> GARLQEIYNRMDPRAQTPVPGKGPFGREELLRRKLIHDGCLLWKTATGRFKDVLVLLMTDVLVFLQEKDQKYIFPTLDKPSVVSLQNLIVRDIANQEKGMFLISAAPPEMYEVHTASRDDRSTW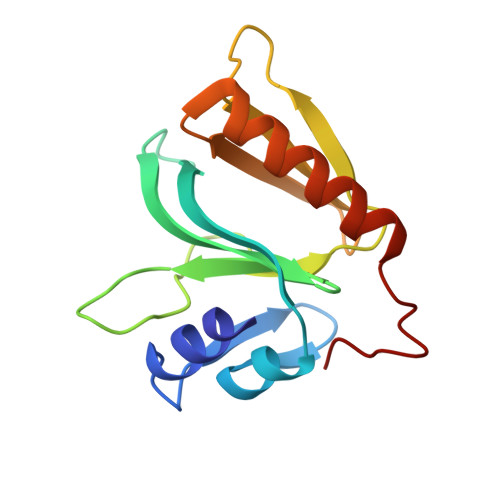IRVIQQSVRTCPSREDFPLI> KDINNNVE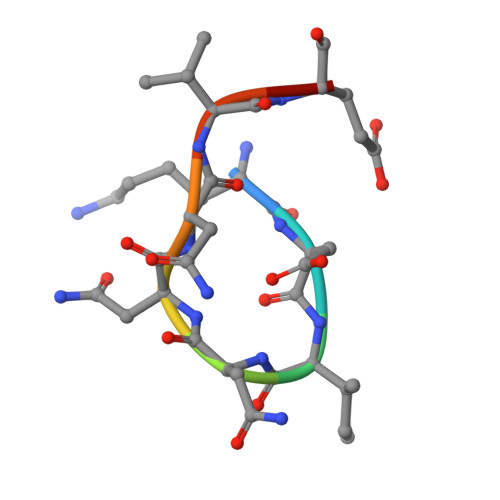K>MRGSHHHHHHGMASHMSSKLVLVLNCGSSSLKFAIIDAVNGDEYLSGLAECFHLPEARIKWKMDGSKQEAALGAGAAHSEALNFIVNTILAQKPELSAQLTAIGHRIVHGGEKYTSSVVIDESVIQGIKDSASFAPLHNPAHLIGIAEALKSFPQLKDKNVAVFDTAFHQTMPEESYLYALPYSLYKEHGVRRYGAHGTSHFYVTQEAAKMLNKPVEELNIITCHLGNGGSVSAIRNGKCVDTSMGLTPLEGLVMGTRSGDIDPAIIFHLHDTLGMSVDQINKMLTKESGLLGLTEVTSDCRYVEDNYATKEDAKRAMD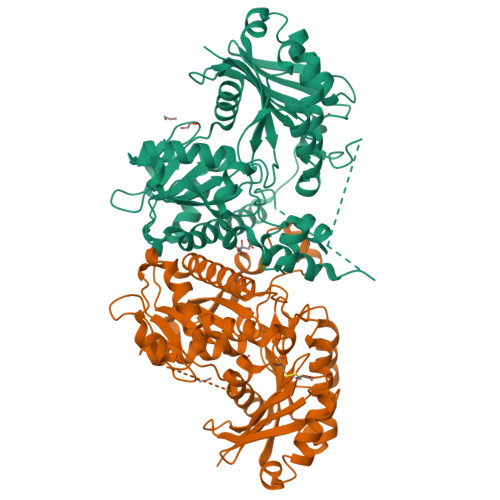VYCHRLAKYIGSYTALMDGRLDAVVFTGGIGENAAMVRELSLGKLGVLGFEVDHERNLAARFGKSGFINKEGTRPAVVIPTNEELVIAQDASRLTA[2x]> RTKSWTDDLKVCNQTGVGEAINQIYKDDGRRCEGYESRDKKCLCISDNNTSLYAILSGHNGVTVAENALQEMAAELLLGQLNVCNTDEAVKELIRQSFMSVEKGYF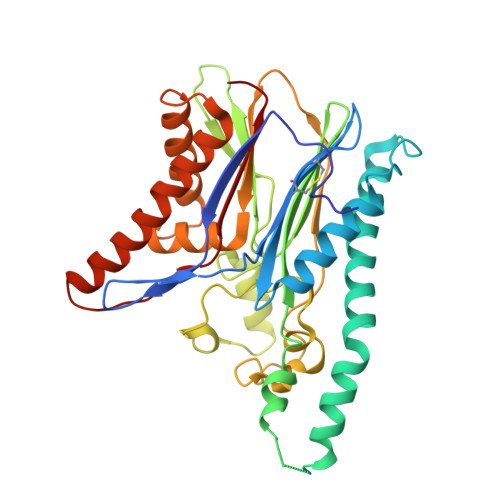DSINPHVATKTAIQLHLSADGMNQYEISQQFENVLQKLDSLNNALSVGSSAVLALIHRSHLYLGNIGNCRALLCKTDEHDTLTVTQLSVDHNLLNAEEAARLFRLGLMAQNFEGVPLYSTRCIGNYLGKAGYKDCNFLSSATAEPVIFEPEIVGGIQITPACRFLVLMSSGLCRALHEIFPGDASTGNRELVRMISEEFQNQSTLGGVAQSVVHRIVQAHHDTYMQLVEEHRSVTFNSRDDVTLLIRNFNYA> MTARRFLNELADLYGVATSYTDYKGAHIEVSDDTLVKILRALGVNLDTSNLPNDDAIQRQIALFHDREFTRPLPPSVVAVEGDELVFPVHVHDGSPADVHIELEDGTQRDVSQVENWTAPREIDGIRWGEASFKIPGDLPLGWHKLHLKSNERSAECGLIITPARLSTADKYLDSPRSGVMAQIYSVRSTLSWGMGDFNDLGNLASVVAQDGADFLLINPMHAAEPLPPTEDSPYLPTTRRFINPIYIRVEDIPEFNQLEIDLRDDIAEMAAEFRERNLTSDIIERNDVYAAKLQVLRAIFEMPRSSEREANFVSFVQREGQGLIDFATWC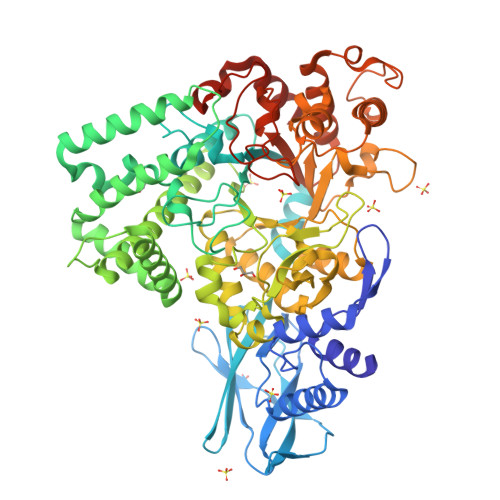ADRETAQSESVHGTEPDRDELTMFYMWLQWLCDEQLAAAQKRAVDAGMSIGIMADLAVGVHPGGADAQNLSHVLAPDASVGAPPDGYNQQGQDWSQPPWHPVRLAEEGYIPWRNLLRTVLRHSGGIRVDHVLGLFRLFVMPRMQSPATGTYIRFDHNALVGILALEAELAGAVVIGEDLGTFEPWVQDALAQRGIMGTSILWFEHSPSQPGPRRQEEYRPLALTTVTTHDLPPTAGYLEGEHIALRERLGVLNTDPAAELAEDLQWQAEILDVAASANALPAREYVGLERDQRGELAELLEGLHTFVAKTPSALTCVCLVDMVGEKRAQNQPGTTRDMYPNWCIPLCDSEGNSVLIESLRENELYHRVAKASKRDLEHHHHHH> PISPIETVPVKLKPGMDGPKVKQWPLTEEKIKALVEICTEMEKEGKISKIGPENPYNTPVFAIKKKDSTKWRKLVDFRELNKRTQDFWEVQLGIPHPAGLKKKKSVTVLDVGDAYFSVPLDEDFRKYTAFTIPSINNETPGIR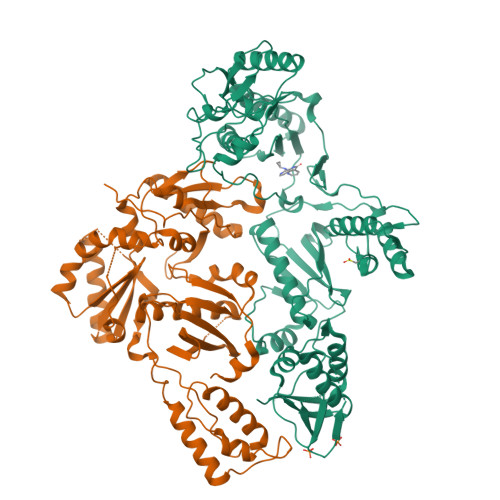YQYNVLPQGWKGSPAIFQSSMTKILEPFRKQNPDIVIYQYVDDLYVGSDLEIGQHRTKIEELRQHLLRWGLTTPDKKHQKEPPFLWMGYELHPDKWTVQPIVLPEKDSWTVNDIQKLVGKLNWASQIYPGIKVRQLCKLLRGTKALTEVIPLTEEAELELAENREILKEPVHGVYYDPSKDLIAEIQKQGQGQWTYQIYQEPFKNLKTGKYARMRGAHTNDVKQLTEAVQKITTESIVIWGKTPKFKLPIQKETWETWWTEYWQATWIPEWEFVNTPPLVKLWYQLEKEPIVGAETFYVDGAANRETKLGKAGYVTNRGRQKVVTLTDTTNQKTELQAIYLALQDSGLEVNIVTDSQYALGIIQAQPDQSESELVNQIIEQLIKKEKVYLAWVPAHKGIGGNEQVDKLVSAGIRKVL;> PISPIETVPVKLKPGMDGPKVKQWPLTEEKIKALVEICTEMEKEGKISKIGPENPYNTPVFAIKKKDSTKWRKLVDFRELNKRTQDFWEVQLGIPHPAGLKKKKSVTVLDVGDAYFSVPLDEDFRKYTAFTIPSINNETPGIRYQYNVLPQGWKGSPAIFQSSMTKILEPFRKQNPDIVIYQYVDDLYVGSDLEIGQHRTKIEELRQHLLRWGLTTPDKKHQKEPPFLWMGYELHPDKWTVQPIVLPEKDSWTVNDIQKLVGKLNWASQIYPGIKVRQLCKLLRGTKALTEVIPLTEEAELELAENREILKEPVHGVYYDPSKDLIAEIQKQGQGQWTYQIYQEPFKNLKTGKYARMRGAHTNDVKQLTEAVQKITTESIVIWGKTPKFKLPIQKETWETWWTEYWQATWIPEWEFVNTPPLVKLWYQLEKEPIVGAETF>[4x]MACLSRIDANLLQYYEKPEPNNTVDLYVSNNSNNNGLKEGDKSISTPVPQPYGSEYSNCLLLSNSEYICYHFSSRSTLLTFYPLSDAYHGKTINIHLPNASMNQRYTLTIQEVEQQLLVNVILKDGSFLTLQLPLSFLFSSANTLNGEWFHLQNPYDFTVRVPHFLFYVSPQFSVVFLEDGGLLGLKKVDGVHYEPLLFNDNSYLKCLTRFFSRSSKSDYDSVISCKLFHERYLIVLTQNCHLKIWDLTSFTLIQDYDMVSQSDSDPSHFRKVEAVGEYLSLYNNTLVTLLPLENGLFQMGTLLVDSSGILTYTFQNNIPTNLSASAIWSIVDLVLTRPLELNVEASYLNLIVLWKSGTASKLQILNVNDESFKNYEWIESVNKSLVDLQSEHDLDIVTKTGDVERGFCNLKSRYGTQIFERAQQILSENKIIMAHN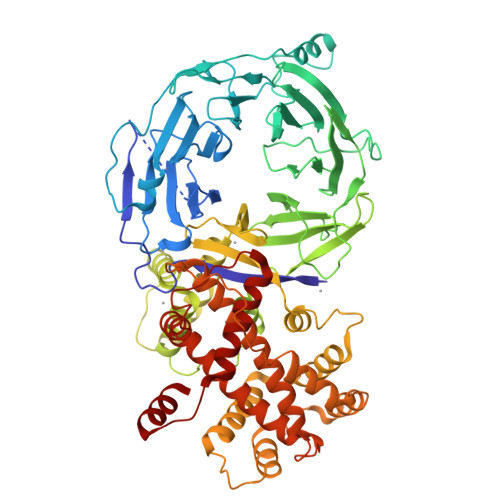EDEEYLANLETILRDVKTAFNEASSITLYGDEIILVNCFQPYNHSLYKLNTTVENWFYNMHSETDGSELFKYLRTLNGFASTLSNDVLRSISKKFLDIITGELPDSMTTVEKFTDIFKNCLENQFEITNLKILFDELNSFDIPVVLNDLINNQMKPGIFWKKDFISAIKFDGFTSIISLESLHQLLSIHYRITLQVLLTFVLFDLDTEIFGQHISTLLDLHYKQFLLLNLYRQDKCLLAEVLLKDSSEFSFGVKFFNYGQLIAYIDSLNSNVYNASITENSFFMTFFRSYII> GSAMARTEKIYIYGASGHGLVCEDVAKNMGYKECIFLDDFKGMKFESTLPKYDFFIAIGNNEIRKKIYQKISENGFKIVNLIHKSALISPSAIVEENAGILIMPYVVINAKAKIEKGVILNTSSVIEHECVIGEFSHVSVGAKCAGNVKIGKNCFLGINSCVLPNLSLADDSILGGGATLVKNQDEK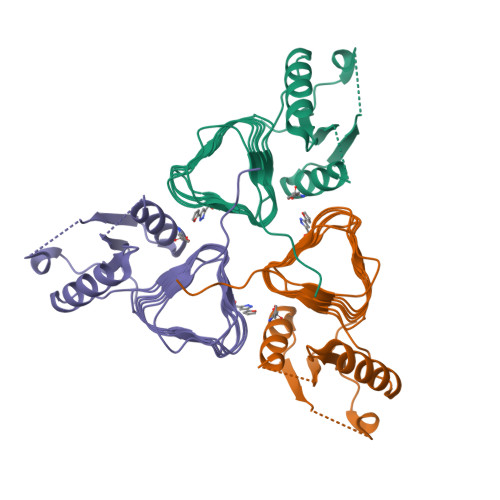GVFVGVPAKRM Here we report the discovery of type IV borosin natural product pathways (termed ‘split borosins’), featuring an iteratively acting α-N-methyltransferase and separate precursor peptide substrate from the metal-respiring bacterium Shewanella oneidensis. The α-N-methyltransferase SonM from Shewanella oneidensis MR-1 iteratively methylates its substrate SonA at two residues, SonA-L63 and SonA-I65, in an N-to-C terminal fashion on the core peptide. Complexes of SonM and SonA form dimers of heterodimers. A five helical bundle at the N-terminus of SonA, now referred to as the borosin binding domain (BBD; 1–53), serves as the SonA leader peptide and is homologous to a portion of the fused clasp region of OphMA.

Mutation of SonM-R67A produced an inactive enzyme, that when co-crystallized with SonA and SAH, was at once unable to maintain normal contacts with the top clamp, while still binding the cofactor in a manner that allowed the bottom lock to close. The resulting SonM-R67A—SonA-0Me—SAH crystal structure complex thus revealed our only structural data of an unmethylated SonA core peptide. In this structure, the bottom lock (the π–π sandwich stacking between SonM-W166 and SonM-F99) is closed, concomitant to the binding of SAH, whereas the top lock is open due to the SonM-R67A mutation. In fact, the structure captures an intermediate conformation between the observed closed conformations (e.g., apo or SAH-bound wt structures) and the open conformation of the SonM—SonA-BBD heterodimer. Interestingly, the core peptide is bound in the active site of SonM as an α-helix (3.5 turns). Concomitantly, helix 5 of the BBD (2.5 turns; as observed in the wt structure) is entirely unwound in the SonM-R67A—SonA-0Me—SAH complex. Comparison between the wt SonM—SonA-2Me—SAH and the SonM-R67A—SonA-0Me—SAH complexes highlights the extent of the change and reveals that unwinding of the BBD’s helix 5 appears necessary to allow the longer section of the core peptide (SonA 53–71 of SonM-R67A—SonA-0Me—SAH vs. SonA 62–71 of wt) to enter the active site in the form of an α-helix. In contrast to all previously described structures, the SonM-R67A—SonA-0Me—SAH structure is not a post-reaction complex. We note that the structure is a pre-reaction complex but is not in a productive conformation: the closest core peptide backbone NH group to the sulfur atom of SAH is “i−9” (6.4 Å). However, the SonM-R67A—SonA-0Me—SAH structure suggests SonM-R67 is critical for the top clamp conformation, core peptide configuration, and the positioning of the complex into productive modes.

>[2x]MGSLVCVGTGLQLAGQISVLSRSYIEHADIVFSLLPDGFSQRWLTKLNPNVINLQQFYAQNGEVKNARDTYEQMVNAILDAVRAGKKTVCALYGHPGVFACVSHMAITRAKAEGFSAKMEPGISAEACLWADLGIDPGNSGHQSFEASQFMFFNHVPDPTTHLLLWQIAIAGEHTLTQFHTSSDRLQILVEQLNQWYPLDHEVVIYEAANLPIQAPRIERLPLANLPQAHLMPISTLLIPPAKKLEYNYAILAKLGIGPEDLG;>[2x]HHMSGLSDFFTQLGQDAQLMEDYKQNPEAVMRAHGLTDEQINAVMTGDMEKLKTLSGDSSYQSYLVISHGNGD>GHMASVTRAVFGELPSGGGTVEKFQLQSDLLRVDIISWGCTITALEVKDRQGRASDVVLGFAELEGYLQK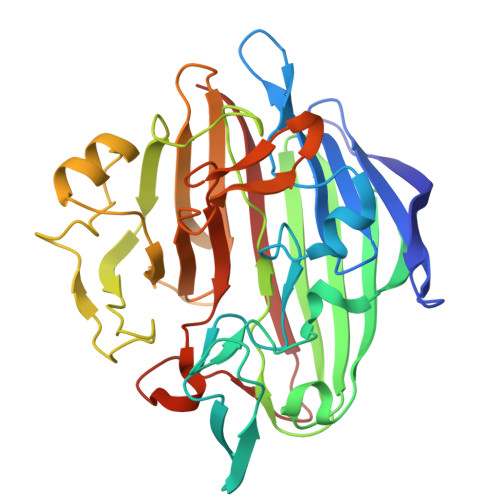QPYFGAVIGRVANRIAKGTFKVDGKEYHLAINKEPNSLHGGVRGFDKVLWTPRVLSNGVQFSRISPDGEEGYPGELKVWVTYTLDGGELIVNYRAQASQATPVNLTNHSYFNLAGQASPNINDHEVTIEADTYLPVDETLIPTGEVAPVQGTAFDLRKPVELGKHLQDFHLNGFDHNFCLKGSKEKHFCARVHHAASGRVLEVYTTQPGVQFYTGNFLDGTLKGKNGAVYPKHSGFCLETQNWPDAVNQPRFPPVLLRPGEEYDHTTWFKFSVA[2x]> KRNKPGKATGKGKPVNNKWLNNAGKDLGSPVPDRIANKLRDKEFKS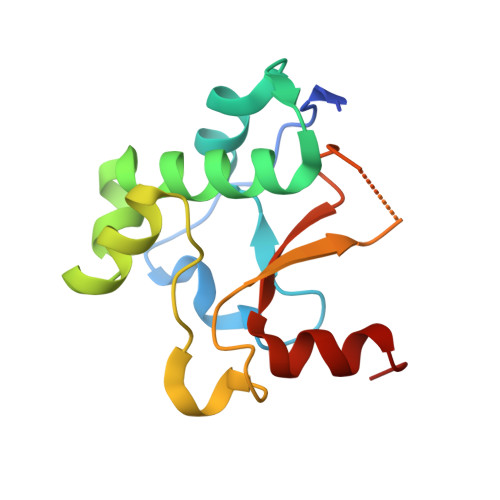FDDFRKKFWEEVSKDPELSKQFSRNNNDRMKVGKAPKTRTQDVSGKRTSFELHHEKPISQNGGVYDMDDISVVTPKRHIDIHRGK>MVRIEVIDIEKPEGVEVIIGQGNFSIFTVDDLARALLTAVPGIKFGIAMNEAKPQLTRYTGNDPELEALAAKNAVKIGAGHVFVILMKNAYPINVLNTIKNHPAVAMIYGASENPFQVIVAETELGR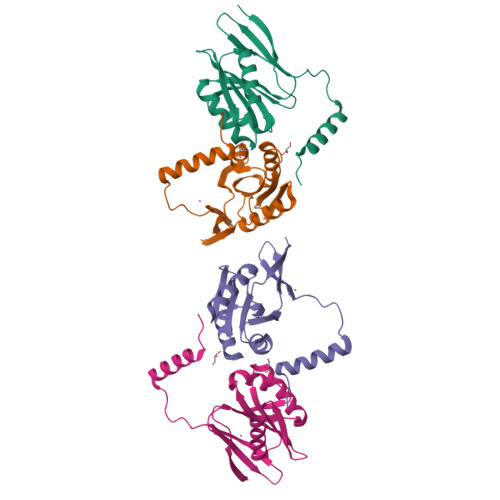AVIGVVDGKAANKIETDEQKKERRELVEKIGYKID[4x]>DSYYQRSDWTADEEQILLGPFDYLES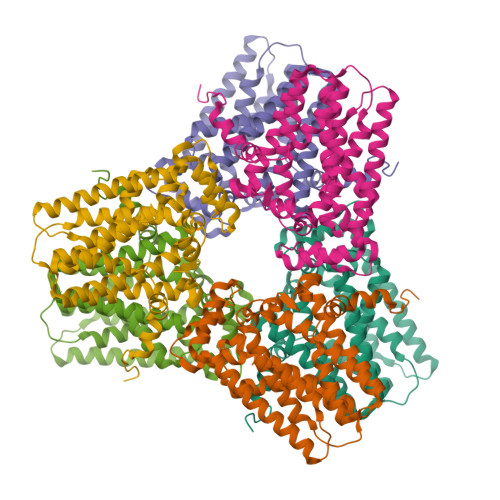LPGKNMRSQLIQSFNTWLKVPTESLDVIIKVISMLHTAFLLIDDIQDQSILRRGQPVAHSIFGTAQAMNSGNYVYFLALREVQKLQNPKAISIYVDSLIDLHRGQGMELFWRDSLMCPTEEQYLDMVANKTGGLFCLAIQLMQAEATIQVDFIPLVRLLGIIFQICDDYLNLKSTAYTDNKGLCEDLTEGKFSFPIIHSIRSNPGNRQLINILKQKPREDDIKRYALSYMESTNSFEYTRGVVRKLKTEAIDTIQGLEKHGLEENIGIRKILARMSLEL[2x]ETHANESULFONIC ACID | C2 H6 O3 S | 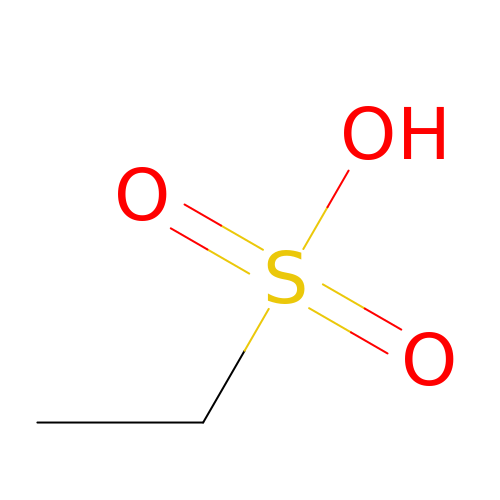CCIVGXIOQKPBKL-UHFFFAOYSA-N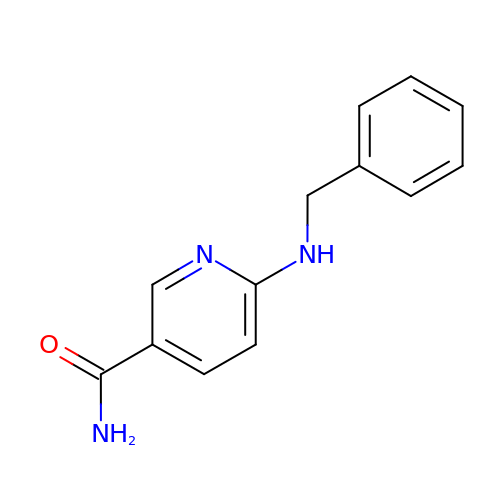6-(benzylamino)pyridine-3-carboxamide | C13 H13 N3 O | JLARFNBDECTDMW-UHFFFAOYSA-N(2Z,4Z)-HEXA-2,4-DIENEDIOIC ACID | C6 H6 O4 | 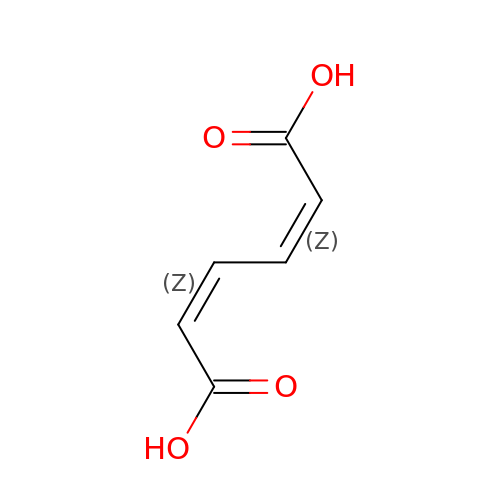TXXHDPDFNKHHGW-CCAGOZQPSA-N> MTTDEGAKNSRGNPAATVAEQGEDVTSKKDRGVLKIVKRVGHGEETPMIGDRVYVHYNGKLANGKKFDSSHDRNEPFVFSIGKGQVIKAWDIGVATMKKGEICHLLCKPEYAYGATGSLPKIPSNATLFFEVELLDFKGEDLLEDGGIIRRTKRRGEGYSNPNEGARVQIHLEGRCGGRVFDCRDVAFTVGEGEDHDIPIGIDKALEKMQREEQCILHLGPRYGFGEAGKPKFGIEPNAELIYEVTLKSFEKAKESWEMDTKEKLEQAAIV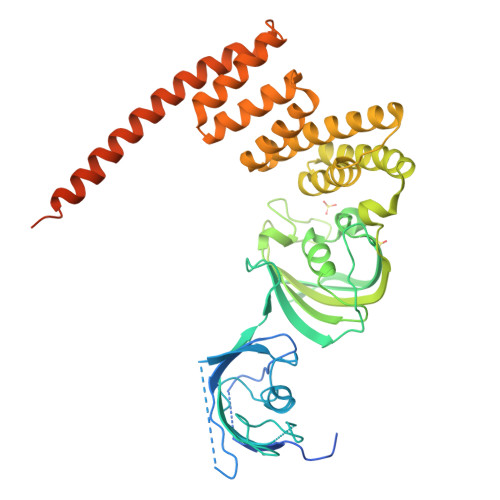KEKGTVYFKGGKYVQAVIQYGKIVSWLEMEYGLSEKESKASESFLLAAFLNLAMCYLKLREYTKAVECCDKALGLDSANEKGLYRRGEAQLLMNEFESAKGDFEKVLEVNPQNKAARLQIFMCQKKAKEHNERDRRTYANMFKKFAEQDAKEEANKAMSKKTSEGVTNEKLTASHAVEEEKPEGHV(2S)-2-amino-5-{[(E)-amino(methylamino)methylidene](hydroxy)azaniumyl}pentanoate 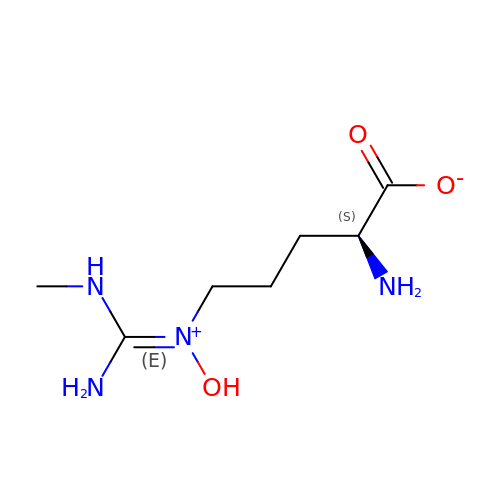| C7 H16 N4 O3 | AZWNHVHYFWVYQE-YFKPBYRVSA-N4-(2-cyclopropyl-7-(6-methylquinolin-5-yl)-1H-benzo[d]imidazol-5-yl)-3,5-dimethylisoxazole | C25 H22 N4 O | 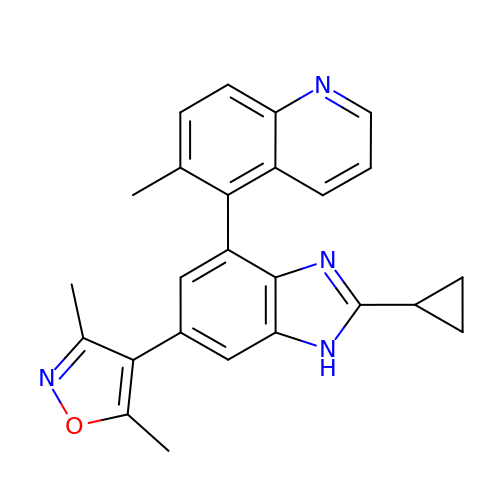KHQQNXFBTALTQF-UHFFFAOYSA-N>[2x]MGSALFLVIFAYLLGSITFGEVIAKLKGVDLRNVGSGNVGATNVTRALGKKYGVLVFFLDFLKGFIPALIAVKSFGIDSWVLTFTG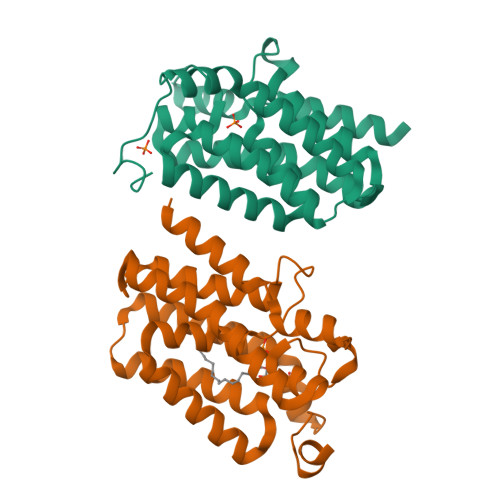LASVLGHMYPVFFGFKGGKGVATALGVVFAVSPSVALFSFLVWLGIFLWKRYVSLASITATISAFLFLFVAGYPVNVLFMAIVIGALIIYRHRENINRLLTGREHRFGTLEVLFQ>SLMEKAARAAKELSRESARAAKELADSNAKAAEDLMREIARSSSSERLLELMAEAIRELQ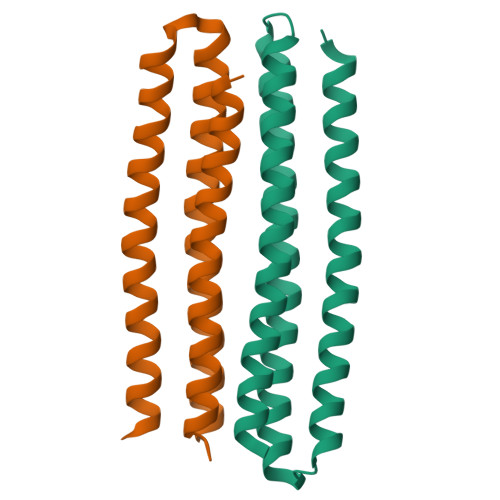KQAAESIADSQRLVVEAIIRLAEAVKQGASEKEIDEIVEEAKKRLEELAERSRQENKKIIDRAKYEMDEESGSLEHHHHHH[6x]>MDSLYDISCFAAGLAGNIFALALFLSPVTTFKRILKAKSTERFDGLPYLFSLLNCLICLWYGLPWVADGRLLVATVNGIGAVFQLAYICLFIFYADSRKTRMKIIGLLVLVVCGFALVSHASVFFFDQPLRQQFVGAVSMASLISMFASPLAVMGVVIRSESVEFMPFYLSLS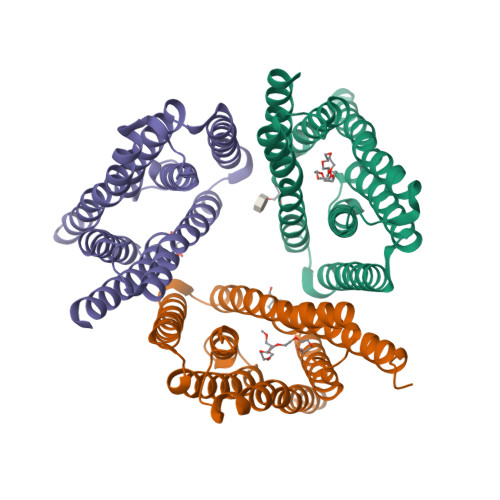TFLMSASFALYGLLLRDFFIYFPNGLGLILGAMQLALYAYYSSNSLEVLFQ[3x]>[2x]AASSPLLIGDSVMVDIGNVFTKKIPNAQIDGKVGRQLVDATPIVKSQYKDYAKKGQKVVVELGTNGAFTKDQLNELLDS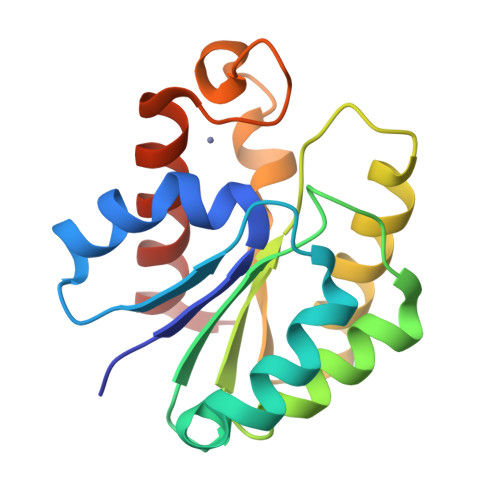FGKADIYLVSIRVPRDYEGRINKLIYEAAAARSNVHLVDWYKASAGHPEYFAYDGIHLEYAGSKALTDLIVKTMETHATN>[2x]MGHQNAAVSENQNHDDGAASSPGFKLVGFSKFVRKNPKSDKFKVKRFHHIEFWCGDATNVARRFSWGLGMRFSAKSDLSTGNMVHASYLLTSGDLRFLFTAPYSPSLSAGEIKPTTTASIPSFDHGSCRSFFSSHGLGVRAVAIEVEDAESAFSISVANGAIPSSPPI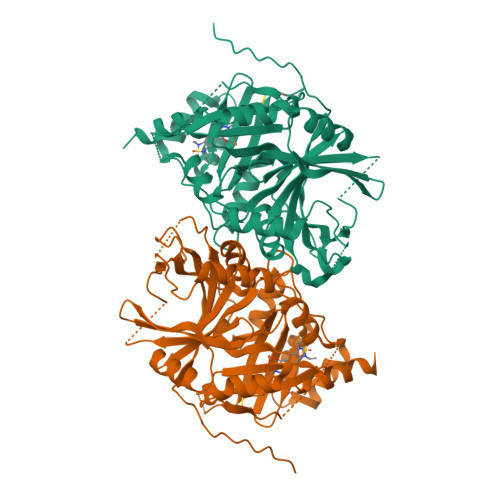VLNEAVTIAEVKLYGDVVLRYVSYKAEDTEKSEFLPGFERVEDASSFPLDYGIRRLDHAVGNVPELGPALTYVAGFTGFHQFAEFTADDVGTAESGLNSAVLASNDEMVLLPINEPVHGTKRKSQIQTYLEHNEGAGLQHLALMSEDIFRTLREMRKRSSIGGFDFMPSPPPTYYQNLKKRVGDVLSDDQIKECEELGILVDRDDQGTLLQIFTKPLGDRPTIFIEIIQRVGCMMKDEEGKAYQSGGCGGFGKGNFSELFKSIEEYEKTLEAKQLVG>[3x]GPLGSPEFSKRSSDPSPAGDNEIERVFVWDLDETIIIFHSLLTGTFASRYGKDTTTSVRIGLMMEEMIFNLADTHLFFNDLEDCDQIHVDDVSSDDNGQDLSTYNFSADGFHSSAPGANLCLGSGVHGGVDWMRKLAFRYRRVKEMYNTYKNNVGG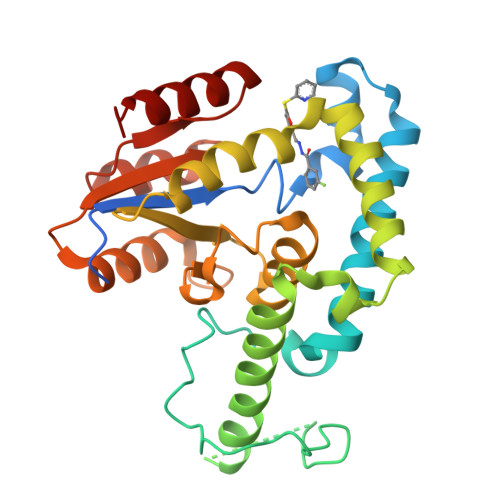LIGTPKRETWLQLRAELEALTDLWLTHSLKALNLINSRPNCVNVLVTTTQLIPALAKVLLYGLGSVFPIENIYSATKTGKESCFERIMQRFGRKAVYVVIGDGVEEEQGAKKHNMPFWRISCHADLEALRHALELEYL>[2x]MAILDSAGVTTVTENGGGEFVDLDRLRRRKSRSDSSNGLLLSGSDNNSPSDDVGAPADVRDRIDSVVNDDAQGTANLAGDNNGGGDNNGGGRGGGEGRGNADATFTYRPSVPAHRRARESPLSSDAIFKQSHAGLFNLCVVVLIAVNSRLIIENLMKYGWLIRTDFWFSSRSLRDWPLFMCCISLSIFPLAAFTV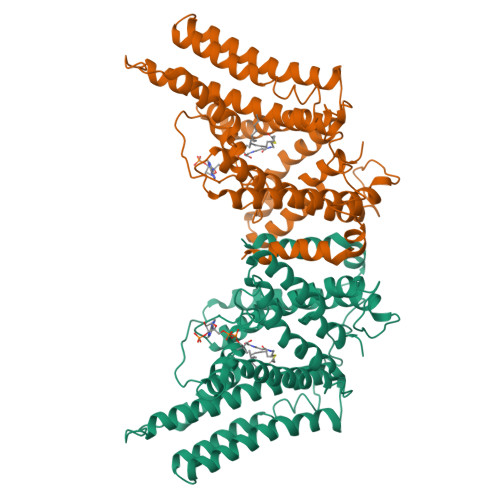EKLVLQKYISEPVVIFLHIIITMTEVLYPVYVTLRCDSAFLSGVTLMLLTCIVWLKLVSYAHTSYDIRSLANAADKANPEVSYYVSLKSLAYFMVAPTLCYQPSYPRSACIRKGWVARQFAKLVIFTGFMGFIIEQYINPIVRNSKHPLKGDLLYAIERVLKLSVPNLYVWLCMFYCFFHLWLNILAELLCFGDREFYKDWWNAKSVGDYWRMWNMPVHKWMVRHIYFPCLRSKIPKTLAIIIAFLVSAVFHELCIAVPCRLFKLWAFLGIMFQVPLVFITNYLQERFGSTVGNMIFWFIFCIFGQPMCVLLYYHDLMNRKGSMSGPHHHHHH>[2x]ARRPTICFRPINPSDLERLEQIHRDIFPIRYESEFFQNVVNGGDIVSWAAVDRSRPD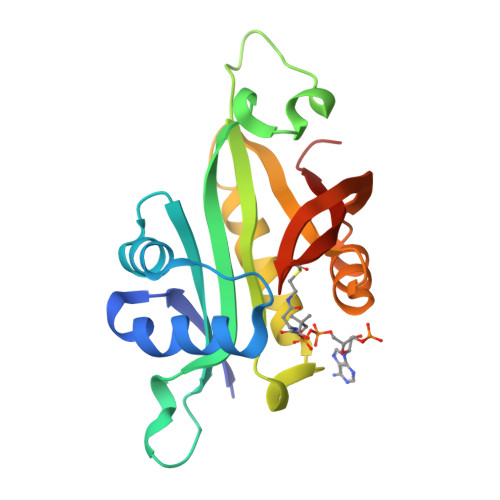GHSEELIGFVTAKIVLAKESEISDLIRYDSSKGEGTLVYILTLGVVETYRKRGIAKALINEVVKYSSGIPVCRGVYLHVIAHNNPAIRLYKRMSFRCVRRLHGFYLINGQHFDSYLFVYFINGS> SIVTKSIVNADAEARYLSPGELDRIKSFVSGGAQRLRIAQVLTDNRERIVKQAGDQLFQKRPDVVSPGGNAYGQEMTATC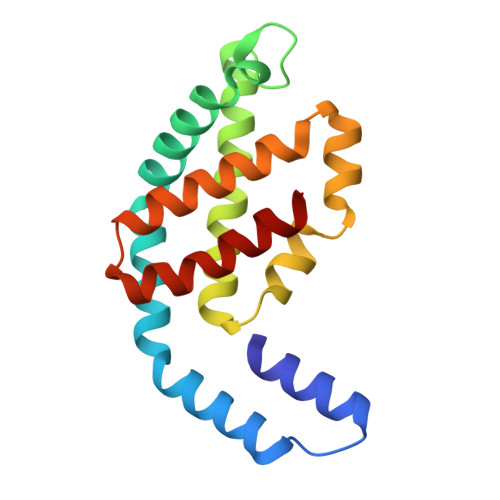LRDLDYYLRLVTYGIVAGDVTPIEEIGIVGVREMYKSLGTPIDAVAGGVAAMKSVAAGLLSAEDAGEAGAYFDYVVGAMQ> PISPIETVPVKLKPGMDGPKVKQWPLTEEKIKALVEICTEMEKEGKISKIGPENPYNTPVFAIKKKDSTKWRKLVDFRELNKRTQDFWEVQLGIPHPAGLKKKKSVTVLDVGDAYFSVPLDEDFRKYTAFTIPSINNETPGIRYQYNVLPQGWKGSPAIFQSSMTKILEPFRKQNPDIVIYQYMDDLCVGSDLEIGQHRTKIEELRQHLLRWGLTTPDKKHQKEPPFLWMGYELHPDKWTVQPIVLPEKDSWTVNDIQKLVGKLNWASQIYPGIKVRQLCKLLRGTKALTEVIPLTEEAELELAENREILKEPVHGVYYDPSKDLIAEIQKQGQGQWTYQIYQEPFKNLKTGKYARMRGAHTNDVKQLTEAVQKITTESIVIWGKTPKFKLPIQKETWETWWTEYWQATWIPEWEFVNTP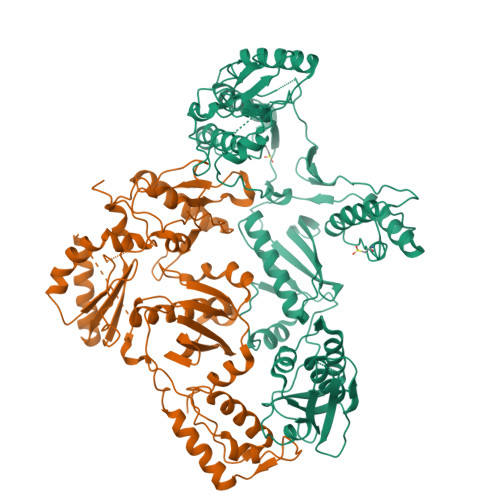PLVKLWYQLEKEPIVGAETFYVDGAANRETKLGKAGYVTNRGRQKVVTLTDTTNQKTELQAIYLALQDSGLEVNIVTDSQYALGIIQAQPDQSESELVNQIIEQLIKKEKVYLAWVPAHKGIGGNEQVDKLVSAGIRKVL;> PISPIETVPVKLKPGMDGPKVKQWPLTEEKIKALVEICTEMEKEGKISKIGPENPYNTPVFAIKKKDSTKWRKLVDFRELNKRTQDFWEVQLGIPHPAGLKKKKSVTVLDVGDAYFSVPLDEDFRKYTAFTIPSINNETPGIRYQYNVLPQGWKGSPAIFQSSMTKILEPFRKQNPDIVIYQYMDDLCVGSDLEIGQHRTKIEELRQHLLRWGLTTPDKKHQKEPPFLWMGYELHPDKWTVQPIVLPEKDSWTVNDIQKLVGKLNWASQIYPGIKVRQLCKLLRGTKALTEVIPLTEEAELELAENREILKEPVHGVYYDPSKDLIAEIQKQGQGQWTYQIYQEPFKNLKTGKYARMRGAHTNDVKQLTEAVQKITTESIVIWGKTPKFKLPIQKETWETWWTEYWQATWIPEWEFVNTPPLVKLWYQLEKEPIVGAETF> MAWDLKVKMLGGNDFLVSVTNSMTVSELKKQIAQKIGVPAFQQRLAHQTAVLQDGLTLSSLGLGPSSTVMLVVQNCSEPLSILVRNERGHSNIYEVFLTQTVDTLKKKVSQREQVHEDQFWLSFEGRPMEDKELLGEYGLKPQCTVIKHLRLR;> MADNMTTTQIEVGPGATNATINFEAGILECYERFSW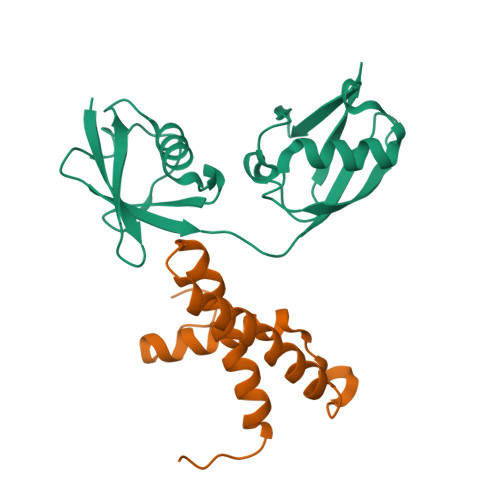QRALDYPGQDRLHRLKRKLESRIKTHNKSEPENKRMSLEERKAIGVKMMKVLLFMDPSAGIEGFEPY> GPLGSPEFMNKQWYLLANQLILSLSKYEGGHIFEKLVDAKKQNCPDYYDVIKNPMSFSCIKTKLKKGQYAYPSEFVKDVQLIFDNCSLYNTSNSVV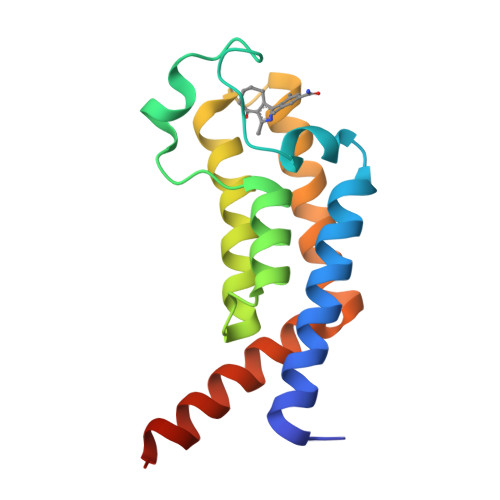AITGKNIETYFNNQLIVMGYNNFILKEKKINDMLKLVEEEN> MALARPRPRLGDLIEISRFGYAHWAIYVGDGYVVHLAPASEIAGAGAASVLSALTNKAIVKKELLSVVAGGDNYRVNNKHD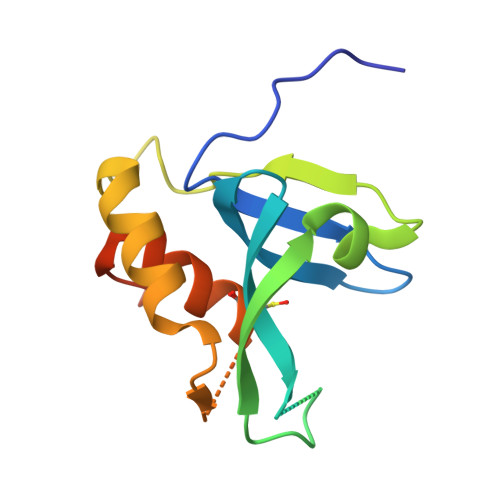DRYTPLPSNKIVKRAEELVGQELPYSLTSDNCEHFVNHLRYGVSRSDQLEHHHHHH> MGSDKIHHHHHHMSDSLVVCEVDPELK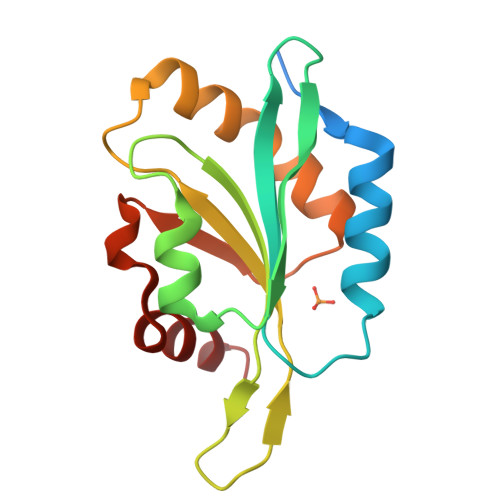ETLRKFRFRKETNNAAIIMKVDKDRQMVVLEDELQNISPEELKLELPERQPRFVVYSYKYVHDDGRVSYPLCFIFSSPVGCKPEQQMMYAGSKNRLVQTAELTKVFEIRTTDDLTETWLKEKLAFFR> GSHMGTVWVTDHGNNRVVKLAAGSNTQTVLPFTGLNTPSGVAVDSAGTVWVTDHGNNRVVKLAAGSNTQTVLPFTGLNTPSGVAVDSAGTVWVTDHGNNRVVKLAAGSNTQTVLPFTGLNTPSGVAVDSAGTVWVTDHGNNRVVKLAAGSNTQTVLPFTGLNTPSGVAVDSAGTVWVTDHGNNRVVKLA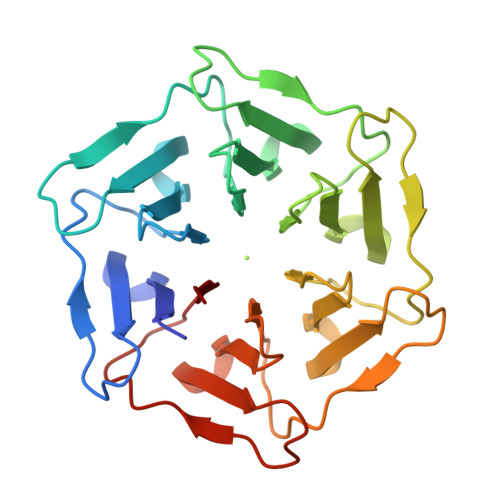AGSNTQTVLPFTGLNTPSGVAVDSAGTVWVTDHGNNRVVKLAAGSNTQTVLPFTGLNTPSGVAVDS>GHMMKRALTGIQASGKQHLGNYLGVMQSLIELQEQCQLFVFVADLHSITVDFQPQALKQNNFDLVRTLLAVGLDPQKACLFLQSDLLEHSMMGYLMMVQSNLGELQRMTQFKAKKAEQTRNPNGTLNIPTGLLTYPALMAGDILLYQPDIVPVGNDQKQHLELTRDLAQRIQKKFKLKLRLPQFVQNKDTNRIMDLFDPTKKMSKSSKNQNGVIYLDDPKEVVVKKIRQATTDSFNKIRFASKTQPGVTNMLTILKALLKEPVNQSLTNQLGNDLEAYFSTKSYLDLKNALTEATVNLLVNIQRKREQISREQVFNCLQAGKNQAQATARTTLALFYDGFGL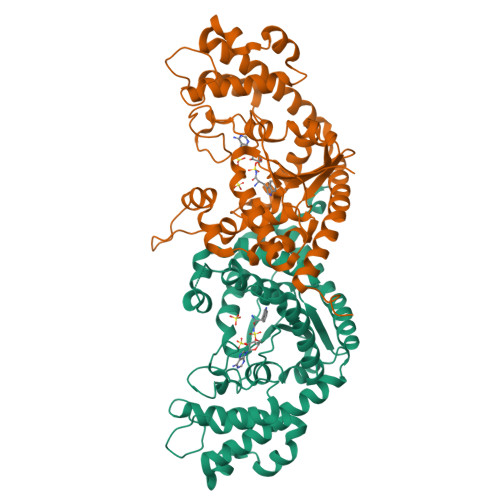GSQNIK[4x]> GPMGNGMNKILPGLYIGNFKDARDAEQLSKNKVTHILSVHDSARPMLEGVKYLCIPAADSPSQNLTRHFKESIKFIHECRLRGESCLVHCLAGVSRSVTLVIAYIMTVTDFGWEDALHTV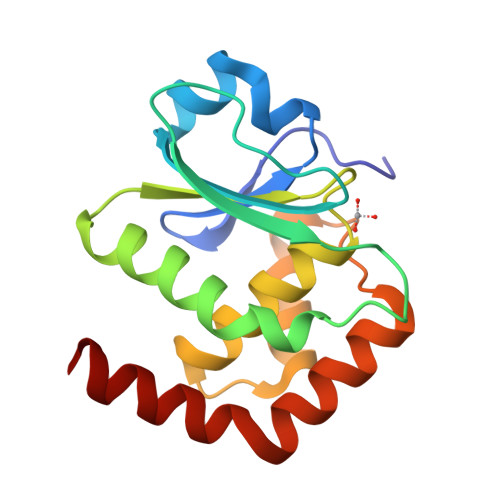RAGRSCANPNVGFQRQLQEFEKHEVHQYRQWLKEEYG> EAFLLFSRRADIRRISLETNNNNVAIPLTGVKEASALDFDVTDNRIYWTDISLKTISRAFMNGSALEHVVEFGLDYPEGMAVDWLGKNLYWADTGTNRIEVSKLDGQHRQVLVWKDLDSPRALALDPAEGFMYWTEWGGKPKIDRAAMDGSERTTLVPNVGRANGLTIDYAKRRLYWTDLDTNLIESSNMLGLNREVIADDLPHPFGLTQYQDYIYWTDWSRRSIERANKTSGQNRTIIQGHLDYVMDILVFHSSRQSGWNECASSNGHCSHLCLAVPVGGFVCGCPAHYSLNADNRTCSAPTTFLLFSQKSAINRMVIDEQQSPDIILPIHSLRN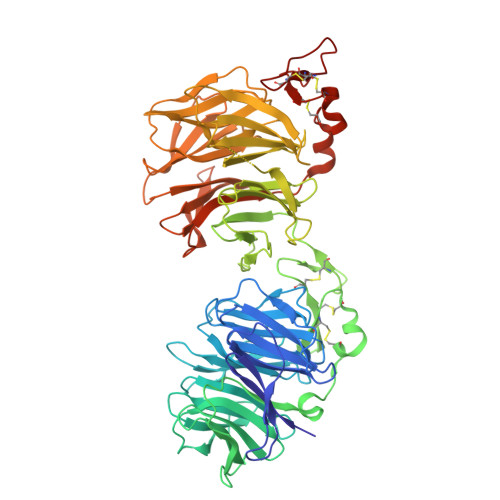VRAIDYDPLDKQLYWIDSRQNMIRKAQEDGSQGFTVVVSSVPSQNLEIQPYDLSIDIYSRYIYWTCEATNVINVTRLDGRSVGVVLKGEQDRPRAIVVNPEKGYMYFTNLQERSPKIERAALDGTEREVLFFSGLSKPIALALDSRLGKLFWADSDLRRIESSDLSGANRIVLEDSNILQPVGLTVFENWLYWIDKQQQMIEKIDMTGREGRTKVQARIAQLSDIHAVKELNLQEYRQHPCAQDNGGCSHICLVKGDGTTRCSCPMHLVLLQDELSCGEP> PTVEE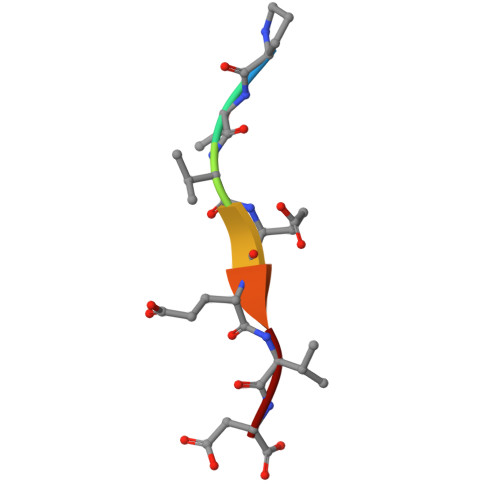VD nitroethane | C2 H5 N O2 | 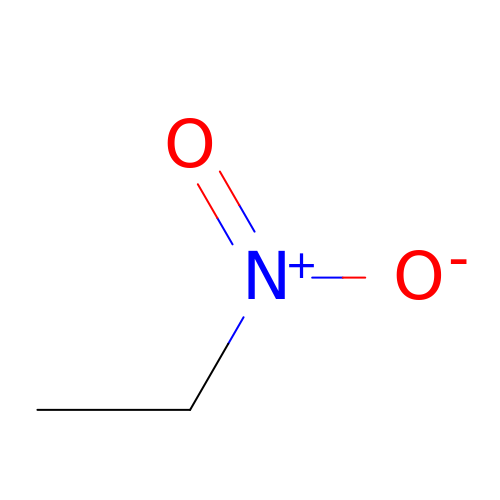MCSAJNNLRCFZED-UHFFFAOYSA-N> GPRPL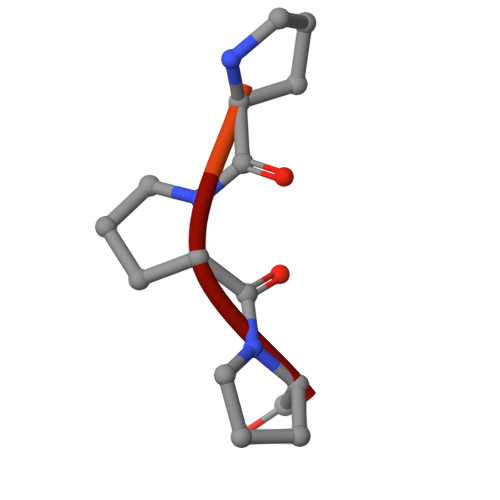PPP> MIVRSFIYEPFQIPSGSMMPTLLIGDFILVEKFAYGIKDPIYQKTLIETGHPKRGDIVVFKYPEDPKLDYIKRAVGLPGDKVTYDPVSKELTIQPGCSSGQACENALPVTYSNVEPSDFVQTFSRRNGGEATSGFFEVPKNETKENGIRLSERKETLGDVTHRILTVPIAQDQVGMYYQQPGQQLATWIVPPGQYFMMGDNRDNSADSRYWGFVPEANLVGRATAIWMSFDK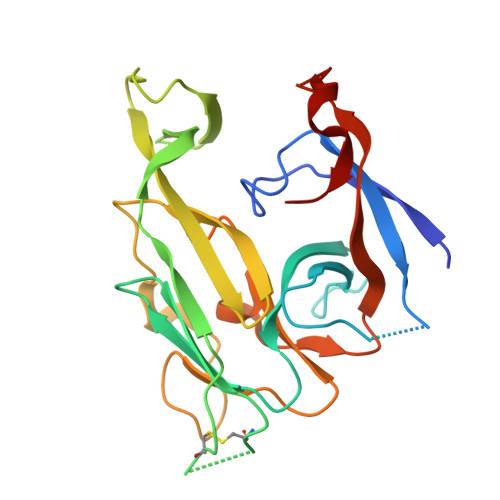QEGEWPTGLRLSRIGGIH> MHREVILCKDQDGKIGLRLKSIDNGIFVQLVQANSPASLVGLRFGDQVLQINGENCAGWSSDKAHKVLKQAFGEKITMTIR

Melanoma differentiation-associated gene 9 (MDA-9) is a small adaptor protein with tandem PDZ domains that promotes tumor progression and metastasis in various human cancers. MDA-9 contains four domains, the N-terminal (1–109aa), PDZ1 (110–193aa), PDZ2 (194–274aa), and the C-terminal (275–298aa). PDZ domains are small, globular PPI domains containing approximately 90 amino acids that form a classical two α-helices (α1, α2) and six β-strands (β1–β6) structure. Through the interactions between the PDZ domains and the substrates, MDA-9 tandem PDZ domains are involved in syndecan-mediated signaling to the cytoskeleton and perform a variety of physiological and cellular functions, e.g., cell–cell adhesion, trans-membrane trafficking, immune regulation, autophagy, ubiquitination, neural development, and exosome control.

Herein, we identified four hits—PI1A, PI1B, PI2A, and PI2B—targeting the PDZ1 and PDZ2 domains of MDA-9, using NMR chemical shift perturbation (CSP). PI1A and PI1B bound to the MDA-9 PDZ1 domain with an affinity of 0.11 and 0.34 mM, respectively, determined from the dose-dependent CSPs. The similar CSP patterns indicated that PI1A and PI1B bound to the same pocket of the MDA-9 PDZ1 domain. To gain insight into the binding details, we solved the crystal structure of the MDA-9 PDZ1 domain in complex with PI1B. The complex structure indicated that PI1B was bound in a typical substrate recognition groove between the α2 helix and β2 strand of the MDA-9 PDZ1 domain. This groove was mainly composed of the residues K124, I125, G126, L127, R128, Q142, H175, and L178. PI1B formed two hydrogen bonds with the backbone of Ile125 and Gly126, and residue G126 was also a conserved residue for binding to the substrate peptide. Notably, the side chains of residues Q142, R128, and K124 were rearranged upon ligand binding, relative to the free form. The cell counting kit-8 (CCK8) assay suggested that PI1A, PI1B, and PI2A were not toxic, while the wound-healing assays demonstrated that PI1A or PI2A alone suppressed the migration of MDA-MB-231 cells. Accordingly, the combination of PI1A and PI2A inhibited migration more effectively than the treatment of a single inhibitor, and PI1B also demonstrated a similar synergetic effect with PI2A.>[2x]SMTFGQALESLKRGHLVAR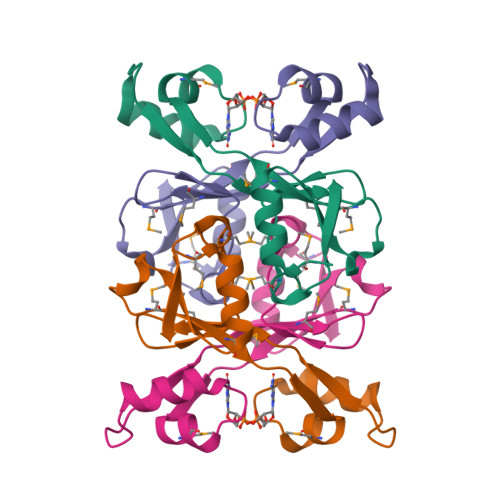KGWNGKGMFIFMRPEDSLPTNMIVNQVKSLPESFKRWVANNHGDSETDRIKFTAYLCMKAADGTIVNGWLASQTDMLANDWVIVE> DYKDDDDKWARGAPRPPPSSPPLSIMGLMPLTKEVAKGSIGRGVLPAVELAIEQIRNESLLRPYFLDLRLYDTECDNAKGLKAFYDAIKYGPNHLMVFGGVCPSVTSIIAESLQGWNLVQLSFAATTPVLADKKKYPYFFRTVPSDNAVNPAILKLLKHYQWKRVGTLTQDVQRFSEVRNDLTGVLYGEDIEISDTESFSNDPCTSVKKLKGNDVRIILGQFDQNMAAKVFCCAYEENMYGSKYQWIIPGWYEPSWWEQVHTEANSSRCLRKNLLAAMEGYIGVDFEPLSSKQIKTISGKTPQQYEREYNNKRSGVGPSKFHGYAYDGIWVIAKTLQRAMETLHASSRHQRIQDFNYTDHTLGRIILNAMNETNFFGVTGQVVFRNGERMGTIKFTQFQDSREVKVGEYNAVADTLEIINDTIRFQGSEPPKDKTIILEQLRKISLPLYSILSALTILGMIMASAFLFFNIKNRNQKLIKMSSPYMNNLIILGGMLSYASIFLFGLDGSFVSEKTFETLCTVRTWILTVGYTTAFGAMFAKTWRVHAIFKNVKMKKKIIKDQKLLVIVGGM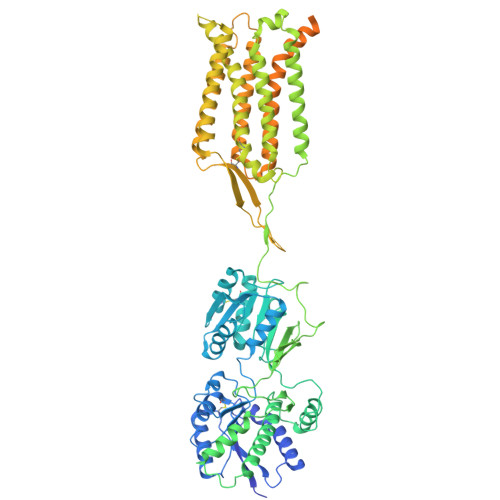LLIDLCILICWQAVDPLRRTVEKYSMEPDPAGRDISIRPLLEHCENTHMTIWLGIVYAYKGLLMLFGCFLAWETRNVSIPALNDSKYIGMSVYNVGIMCIIGAAVSFLTRDQPNVQFCIVALVIIFCSTITLCLVFVPKLITLRTNPDAATQNRRFQFTQNQKKEDSKTSTSVTSVNQASTSRLEGLQSENHRLRMKITELDKDLEEVTMQLQDTPEKTTYIKQNHYQELNDILNLGNFTESTDGGKAILKNHLDQNPQLQWNTTEPSRTCKDPIEDINSPEHIQRRLSLQLPILHHAYLPSIGGVDASCVSPCVSPTASPRHRHVPPSFRVMVSGL We have recently shown that T. vaginalis has acquired NlpC/P60 genes from bacteria, expanding them to a repertoire of nine TvNlpC genes in two distinct clans, and that TvNlpCs of clan A are active against bacterial peptidoglycan. NlpC/P60-containing enzymes typically hydrolyse the stem peptides of bacterial peptidoglycan (PG). We characterized the 3D structure of TvNlpC_B3 alone and with the inhibitor E64 bound, probing the active site of these enzymes for the first time.

The final model of TvNlpC_B3, refined to an R/Rfree of 0.158/0.170 (full data collection and refinement statistics in S2 Table), and contains the contiguous segment from Asn23 to Tyr137. As expected, TvNlpC_B3 exhibits an α+β, papain-like fold, consisting of 4 α-helices and 5 β-sheets arranged in antiparallel fashion. The active site residues of TvNlpC_B3 form a catalytic triad, identified as Cys53, His99 and His111 using homology with family members. Helix2 contains the active site cysteine at the N-terminus of the helix, positioning it in close proximity with His99 and His111. His111 is also responsible for the single unusual rotamer of our model and is supported by well-defined electron density. Similarly to other Cys-His-His peptidases, the positioning of His111 appears to orientate His99 for facilitating enzymatic activity (via hydrogen bonding between ND1 atom of His111 and the NE2 atom of His99). The active site groove runs from the N-terminus of Helix α2, between β-strands 2 and 3 and across the β-sheet ending at strand 4. This groove occupies a full face of the domain, making it a dominant feature of the otherwise globular protein. The active site cysteine is located centrally within the grove, with the imidazole groups of histidine residues on one side, and the hydroxyl of Ser54 on the other, altogether forming the groove’s floor. The serine side of the groove terminates on the R group of the highly conserved Arg71 (where the first SH3b domain of NlpC_A1 would interact with the NlpC/P60 domain).

> GPGHERREVPNASGSAILNVAKSRIGKQYMSGGTGPDLFDCSGLVLYSHNQCGVYGVPRVAKDQARGGKAGSGAAGDVVYFGNPAHHVGICCGDGSMVHAPRPGKTVCILKIAYMKESYGYRRYY>XGEIAKSLKEIAKSLKEIAWSLKEIAKSLKG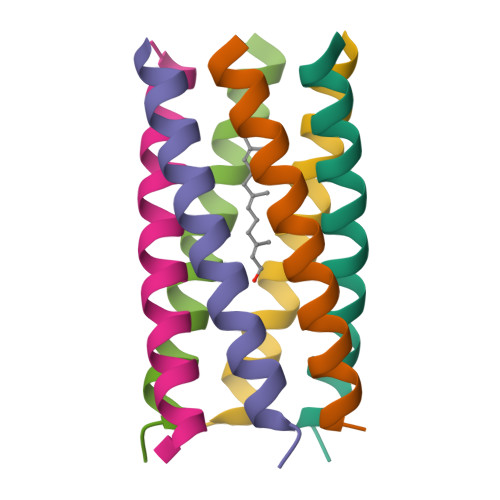X[6x]>[4x]MTDTPFIRPDMKAFLEAIAAMAGPTLAEMTLEEARASYVAL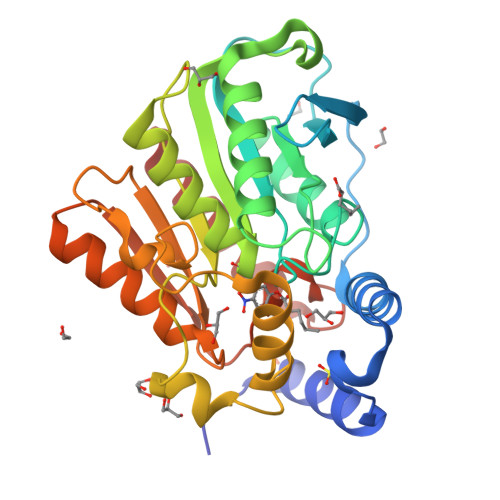HGMADRPARELAVIRNLSCPGPAGDIPLRLYDARESREAGPVITFYHGGGFVIGDLDTHHNLCTEIAALMDLPVVAVDYRLAPEHPFPAAIEDCEAATRWVASSPSELGRTASGVIPIGDSAGGNATIVVSQLLGAKPADVPVVLQVPIFPLASDAVGSASLEAFAEGFVLTKASIEFFDTAYKADRADPRGFPILGDHTAAPPTIVATASLDPIRDSGRDYAKALVEAGRDVVYLEMEGVTHGFTNIRAAVPSTQGDLERIIAAMKMMLGTA2-amino-4-{2,4-dichloro-5-[2-(diethylamino)ethoxy]phenyl}-N-ethylthieno[2,3-d]pyrimidine-6-carboxamide 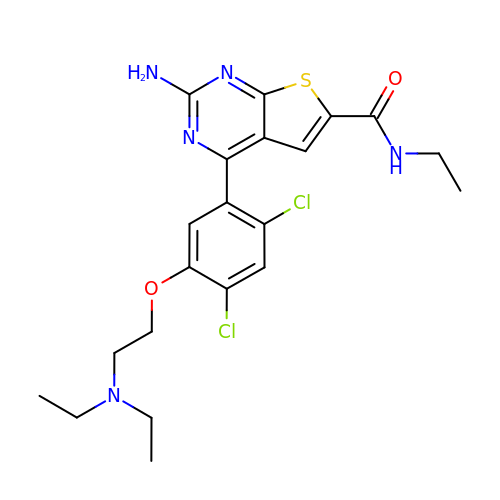| C21 H25 Cl2 N5 O2 S | KQRDVNUCOWRFLN-UHFFFAOYSA-N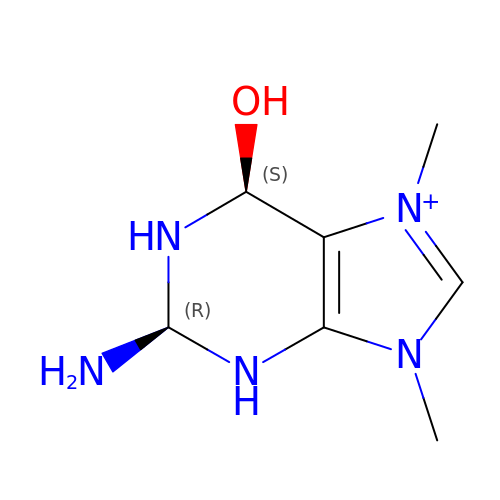7,9-DIMETHYLGUANINE | C7 H14 N5 O | UCYXILDOFXGENE-NKWVEPMBSA-N N-[2-chloro-5-(1-{3-[4-(6-chloro-3-methyl-2-oxo-2,3-dihydro-1H-benzimidazol-1-yl)piperidin-1-yl]propyl}-6-oxo-1,6-dihydropyridazin-3-yl)benzyl]benzamide | C34 H34 Cl2 N6 O3 | 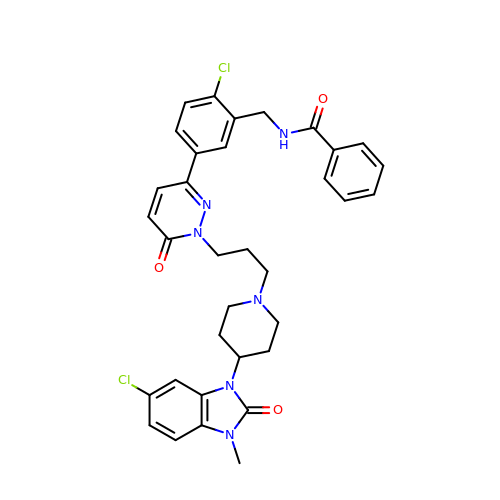ZJXORVFCSQEKCZ-UHFFFAOYSA-N3-[(2-methylbenzyl)sulfanyl]-4H-1,2,4-triazol-4-amine | C10 H12 N4 S | 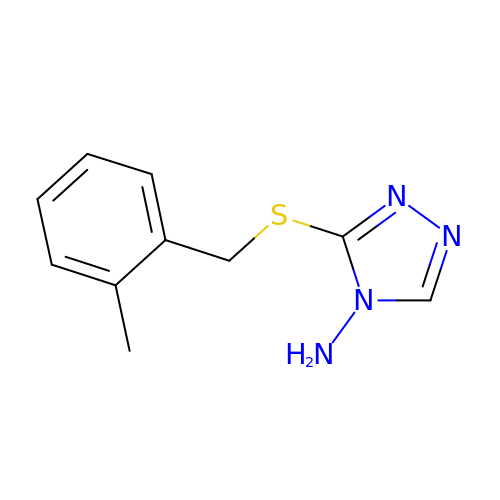UVAUEHMNFBWZNL-UHFFFAOYSA-N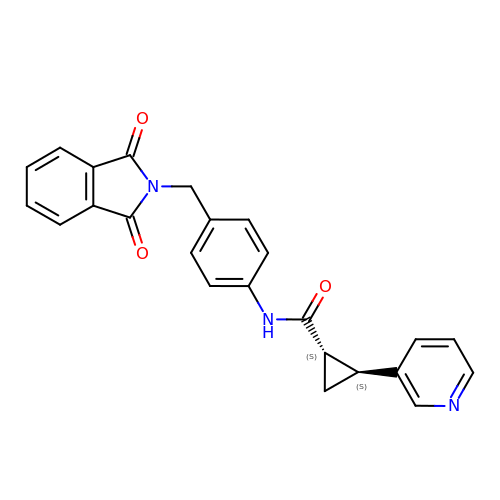(1S,2S)-N-{4-[(1,3-dioxo-1,3-dihydro-2H-isoindol-2-yl)methyl]phenyl}-2-(pyridin-3-yl)cyclopropane-1-carboxamide | C24 H19 N3 O3 | ZFFWKXDUNGUFER-RTWAWAEBSA-N>[8x]MTQPMPGKPAEDAENELDIRGLFRTLWAGKLWIIGMGLAFALIALAYTFFARQEWSSTAITDRPTVNMLGGYYSQQQFLRNLDVRSNMASADQPSVMDEAYKEFVMQLASWDTRREFWLQTDYYKQRMVGNSKADAALLDEMINNIQFIPGDFTRAVNDSVKLIAETAPDANNLLRQYVAFASQRAASHLNDELKGAWAARTIQMKAQVKRQEEVAKAIYDRRMNSIEQALKIAEQHNISRSATDVPAEELPDSEMFLLGRPMLQAALENLQAVGPAFDLDYDQNRAMLNTLNVGPTLDPRFQTYRYLRTPEEPVKRDSPRRAFLMIMWGIVGGLIGAGVALTRRCSKEFRVPGSHHHHHHHH

Lipopolysaccharides such as the enterobacterial common antigen are important components of the enterobacterial cell envelope that act as a protective barrier against the environment and are often polymerized by the inner membrane bound Wzy-dependent pathway. By employing cryo-electron microscopy we show that WzzE, the co-polymerase component of this pathway that is responsible for the length modulation of the enterobacterial common antigen, is octameric with alternating up-down conformations of its L4 loops. The alternating up-down nature of these essential loops, located at the top of the periplasmic bell, are modulated by clashing helical faces between adjacent protomers that flank the L4 loops around the octameric periplasmic bell. This alternating arrangement and a highly negatively charged binding face create a dynamic environment in which the polysaccharide chain is extended, and suggest a ratchet-type mechanism for polysaccharide elongation.

The ConSurf analysis also revealed an arginine within α7 (R267) that interacts with the downward facing L4 to be highly conserved. To investigate how robust the alternating conformation of the L4 loops is, we replaced this residue with an alanine and a glutamic acid in two constructs. Although the change of this amino acid is clearly visible in the cryo-EM density map, replacement had little effect on the overall octameric structure of WzzE or the alternating arrangement of the L4 loops. The R267A variant did, however, have a small, but noticeable 2 Å shift upwards of the entire L4 region suggesting that this conserved residue could somehow help stabilize this otherwise dynamic region of the complex. Although there are only small differences between the native WzzE and both R267 variants, these variants do underscore the nature of the alternating loops in WzzE, as both structures of the mutants were solved independently using reference-free ab-initio starting volumes and clearly display the same pattern of alternating L4 loops in their unsymmetrized C1 maps as the native WzzE.5-PHENYLVALERIC ACID | C11 H14 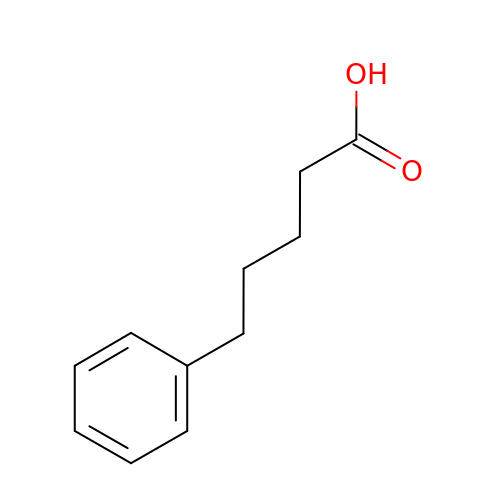O2 | BYHDDXPKOZIZRV-UHFFFAOYSA-N>[6x]MFEIKKICCIGAGYVGGPTCSVIAHMCPEIRVTVVDVNESRINAWNSPTLPIYEPGLKEVVESCRGKNLFFSTNIDDAIKEADLVFISVNTPTKTYGMGKGRAADLKYI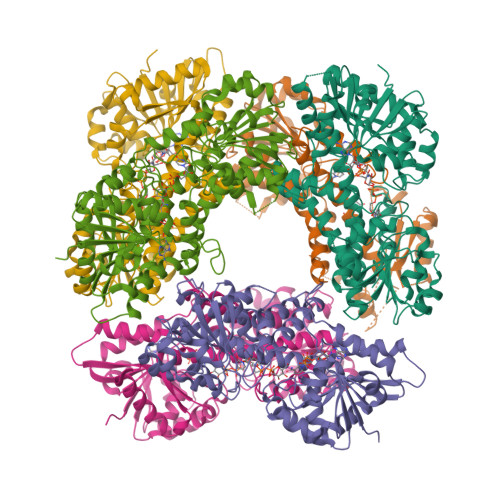EACARRIVQNSNGYKIVTEKSTVPVRAAESIRRIFDANTKPNLNLQVLSNPEFLAEGTAIKDLKNPDRVLIGGDETPEGQRAVQALCAVYEHWVPREKILTTNTWSSELSKLAANLFLAQRISSINSISALCEATGADVEEVATAIGMDQRIGNKFLKASVGFGGSCFQKDVLNLVYLCEALNLPEVARYWQQVIDMNDYQRRRFASRIIDSLFNTVTDKKIAILGFAFKKDTGDTRESSSIYISKYLMDEGAHLHIYDPKVPREQIVVDLSHPGVSEDDQVSRLVTISKDPYEACDGAHAVVICTEWDMFKELDYERIHKKMLKPAFIFDGRRVLDGLHNELQTIGFQIETIGKKVSSKRIPYAPSGEIPKFSLQDPPNKKPKV> MPIELPPTYITPYPEISAGGNGTYRGQDLSSGQSFPRGMQNPVATVLLLQGDLYCSPNCLATFQDQARRDSFGIQSKVALKTFAAADQREAEGRDLRTAYNEIATDIGRSQQINENIIKYPPGNHVLSGGLMTPFHALAHGMFGLGAPLTFPIQNVGLNVDIRGIPDVMNVIQSARPVGTSSLDVNFAYDVGKDSNASWLTLGNITLRLVGTIDKNASGAWTFSGEIRAFNDVYDANPSNHR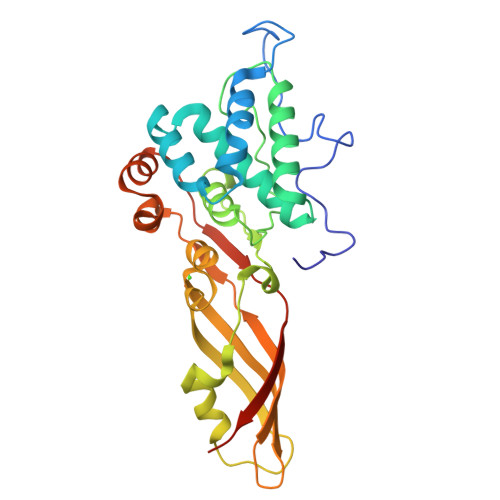GWLGENLTSLLSAVPFTSYSIEIPGSLPVTVSGNLEHHHHHH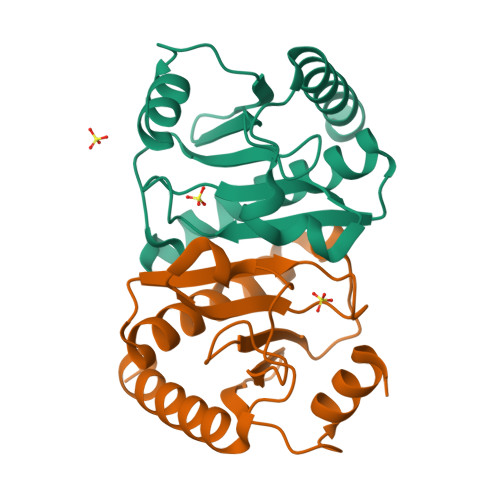>MLMSMATVFTKIINRELPGRFVYEDDDIVAFLTIEPMTQGHTLVVPRAELDNWQDIEPAVFARVMEVSQLIGKAVCKAFDTERSGLIIAGLEVPHLHVHVFPARNLSDFGFANVDRNPSPESLDEAQAKIKAALADLQSAAG[2x]>[4x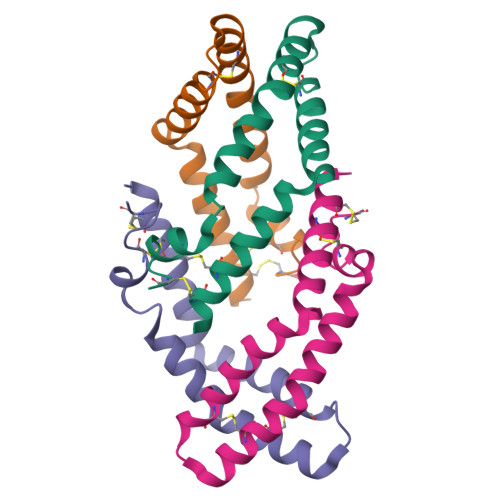]SLPCDICKTVVTEAGNLLKDNATQEEILHYLEKTCEWIHDSSLSASCKEVVDSYLPVILDMIKGEMSNPGEVCSALNLCQSLQ> METFRTLLAKAALGNGISSTAYDTAWVAKLGQLDDELSDLALNWLCERQLPDGSWGAEFPFCYEDRLLSTLAAMISLTSNKHRRRRAAQVEKGLLALKNLTSGAFEGPQLDIKDATVGFELIAPTLMAEAARLGLAICHEESILGELVGVREQKLRKLGGSKINKHITAAFSVELAGQDGVGMLDVDNLQETNGSVKYSPSASAYFALHVKPGDKRALAYISSIIQAGDGGAPAFYQAEIFEIVWSLWNLSRTDIDLSDPEIVRTYLPYLDHVEQHWVRGRGVGWTGN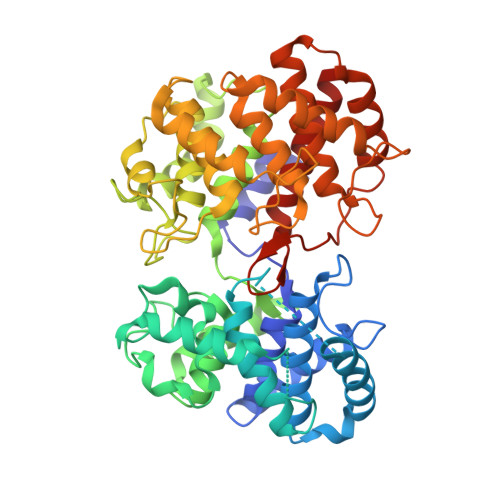STLEDCDTTSVAYDVLSKFGRSPDIGAVLQFEDADWFRTYFHEVGPSISTNVHVLGALKQAGYDKCHPRVRKVLEFIRSSKEPGRFCWRDKWHRSAYYTTAHLICAASNYDDALCSDAIGWILNTQRPDGSWGFFDGQATAEETAYCIQALAHWQRHSGTSLSAQISRAGGWLSQHCEPPYAPLWIAKTLYCSATVVKAAILSALRLVDESNQ EcoKMcrA from Escherichia coli restricts CpG methylated or hydroxymethylated DNA, and may act as a barrier against host DNA. The enzyme consists of a novel N-terminal specificity domain that we term NEco, and a C-terminal catalytic HNH domain. We determined the crystal structures of NEco in complex with fully modified DNA containing three variants of the Y5mCGR EcoKMcrA target sequence: C5mCGG, T5mCGA and T5hmCGA. The structures show that monomeric NEco has two separate pockets for (hydroxy)methyl groups on cytosines, reachable without nucleotide flipping, and reveal the mechanistic basis for the Y5(h)mCGR sequence specificity of EcoKMcrA.

The purified NEco was co-crystallized with 10mer dsDNA with the central C5mCGG, T5mCGA and T5hmCGA sequences. When Y is a cytosine, the N4 atom of the C is about 3.3 Å away from peptide bond between G32 and P33. This distance would be suitable for an NH–π hydrogen bond. The C5mCGG sequence used before for in vivo and in vitro characterization of EcoKMcrA and NEco exhibited ∼7-fold weaker binding. In the EMSA experiment, stable complexes were only observed with the C5mCGG sequence containing oligoduplexes. Here, we used the competition assay to quantify the contributions of the first and second methyl groups in the C5mCGG context. The data indicate an ∼230-fold preference for fully over hemi-methylated DNA and ∼10-fold preference for hemi- over non-methylated DNA. The binding pocket for the (hydroxy)methyl group in the proximal strand is a locally hydrophobic region, formed by the Cβ atom of S30 and a part of K122 (atoms Cα, Cβ and Cγ). The binding pocket for the (hydroxy)methyl group in the distal strand is primarily formed by the indole ring of W31. The protein-DNA complexes in the three NEco structures are highly similar (all atom rmsd between 0.3 and 0.9 Å).

>GHHHHHHEFMHVFDNNGIELKAECSIGEEDGVYGLILESWGPGDRNKDYNIALDYIIERLVDSGVSQVVVYLASSSVRKHMHSLDERKIHPGEYFTLIGNSPRDIRLKMCGYQAYFSRTGRKEIPSGNRTKRILINVPGIYSDSFWASIIRG[2x]> SKRADKKAILELFQTYKEPLGNYIGAEGLQRLFEDIQVDPSDVVTLVLAWKLKASSTCEFSEKEFVEGLANLQVDSLEKLKRKLSSLRKEIEDPSKFRAFYQFVFQYSKEPSQRSLPAETAMALWDVLLRGRFSLLDSWLEFLKNNTHSI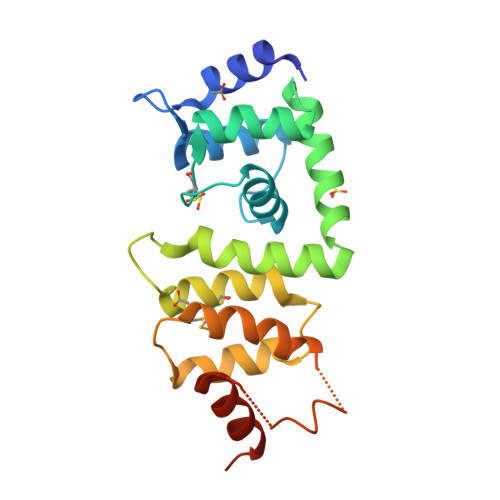SRDTWNLLYDFSQLSEKDLSDYDENGAWPVLIDDFVKWLKHEQPNKHES> GSHMASKPVIRVFILTSNNPELRSRLLLFCLRIVLSNGARDSHRFGALLTMFSLPSATMLNHVKLADQSPEADIERVEIDGFEEGSFRLIPNARSGMSRGEINAYAALAEDLPDTLNHATPFVDSEVEGTAWDEIETFLDMCYSVLMQAWIVTCKCMTAPDQPAASIEKRLQKYRQQGRINPRYLLQPEARRIIQNVIRKGMVVRHFLTFELQLARAQSLVSNRYYAMVGD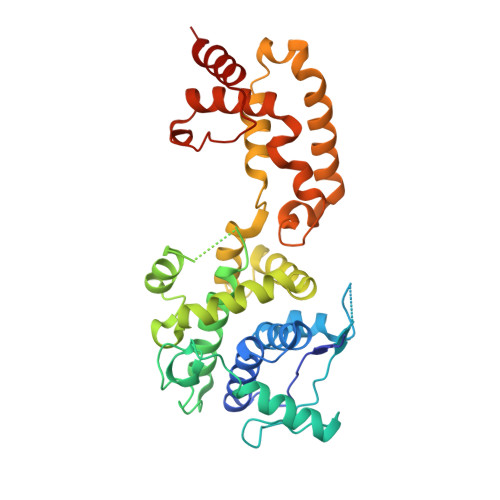VGKYIENCGMGGFFLTLKYALGTRWPTLALAAFSGELTKLKSLMALYQTLGEQARYLALLESPHLMDFAAANYPLLYSYAMGIGYVLDVNMRNYAFSRSYMNKTYFQLGMETARKQM> AACYSSDCRVKCVAMGFSSGKCINSKCK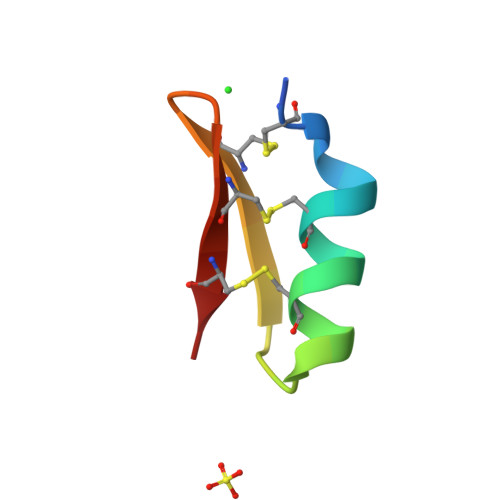CYK>MIVLFVDFDYFYAQVEEVLNPSLKGKPVVVCVFSGRFEDSGAVATANYEARKFGVKAGIPIVEAKKILPNAVYLPMRKEVYQQVSSRIMNLLREYSEKIEIASIDEAYL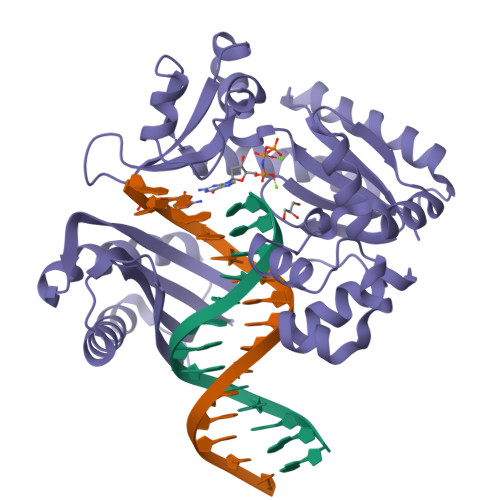DISDKVRDYREAYNLGLEIKNKILEKEKITVTVGISKNKVFAKIAADMAKPNGIKVIDDEEVKRLIRELDIADVPGIGNITAEKLKKLGINKLVDTLSIEFDKLKGMIGEAKAKYLISLARDEYNEPIRTRVRKSIGRIVTMKRNSRNLEEIKPYLFRAIEESYYKLDKRIPKAIHVVAVTEDLDIVSRGRTFPHGISKETAYSESVKLLQKILEEDERKIRRIGVRFSKFI[2x]> EQARPADDALAALGAQLFVDPALSRNATQSCATCHDPARAFTDPREGKAGLAVSVGDDGQSHGDRNTPTLGYAALVPAFHRDANGKYKGGQFWDGRADDLKQQAGQCMLNPVEMAMPDRAAVAARLRDDPAYRTGFEALFGKGVLDDPERAFDAAAEALAAYQATGEFSPFDSKYDRVMRGEEKFTPLEEFGYTVFITWNCRLCHMQRKQ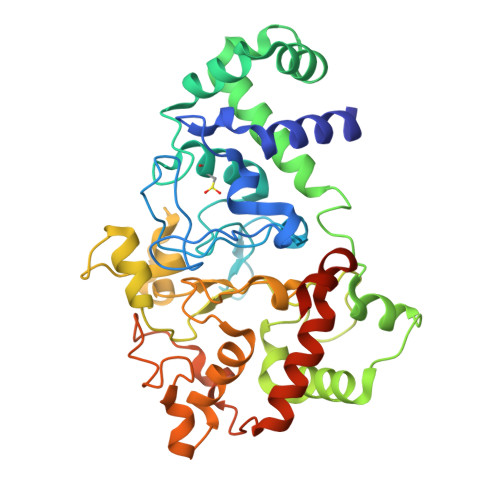GVAERETFTNFEYHNIGLPVNETAREASGLGADHVDHGLLARPGIEDPAQSGRFKVPSLRNVAVTGPYMHNGVFTDLRTAILFYNKYTSRRPEAKINPETGAPWGEPEVARNLSLAELQSGLMLDDGRVDALVAFLETLTDRRYEPLLEESRAAQKDHHHHHH4-[(9-{4-[(E)-2-cyanoethenyl]-2,6-dimethylphenyl}-6-oxo-6,7,8,9-tetrahydro-5H-pyrimido[4,5-b][1,4]diazepin-2-yl)amino]benzonitrile 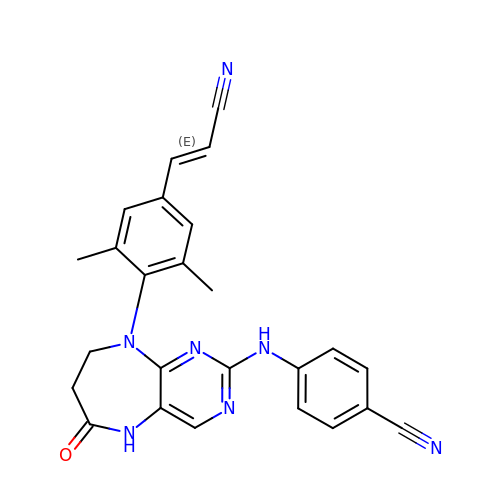| C25 H21 N7 O | CXONFCILERVPJH-ONEGZZNKSA-N> GSGVDFYDVAFKVMLVGDSGVGKTCLLVRFKDGAFLAGTFISTVGIDFRNKVLDVDGVKVKLQMWDTAGQERFRSVTHAYYRDAHALLLLYDVTNKASFDNIQAWLTEIHEYAQHDVALMLLGNKVDSAHERVVKREDGEKLAKEYGLPFMETSAKTGLNVDLAFTAIAKEL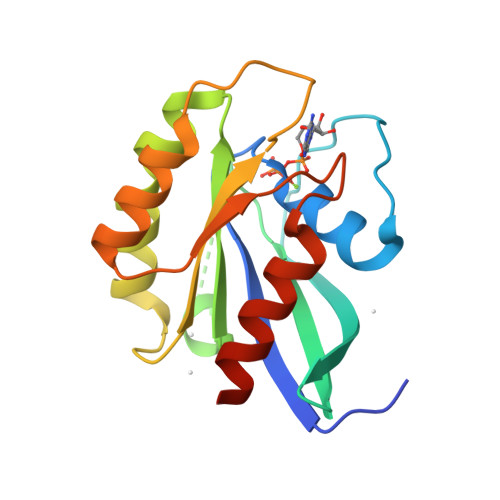KRRSMKAP> SYRPYSYRHFA;> MHHHHHHMQIGWRREGIKYRRNELFLDVLESVNLLMSPQGQVLSAHVSGRVVMKSYLSGMPECKFGMNDKIVIEKQGKGTADETSKSGKQSIAIDDCTFHQCVRLSKFDSERSISFIPPDGEFELMRYRTTKDIILPFRVIPLVREVGRTKLEVKVVIKSNFKPSLLAQKIEVRIP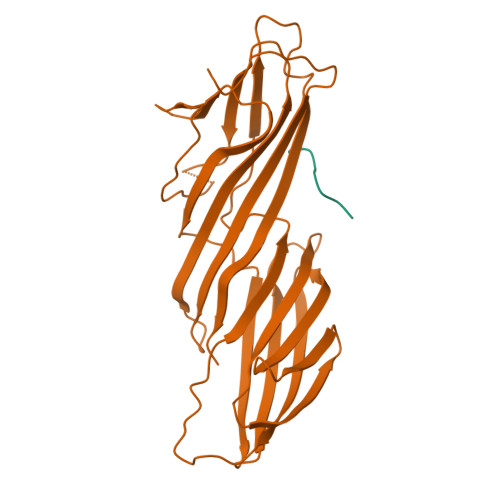TPLNTSGVQVICMKGKAKYKASENAIVWKIKRMAGMKESQISAEIELLPTNDKKKWARPPISMNFEVPFAPSGLKVRYLKVFEPKLNYSDHDVIKWVRYIGRSGIYETRC~{N}-(1~{H}-indazol-5-yl)butane-1-sulfonamide | C11 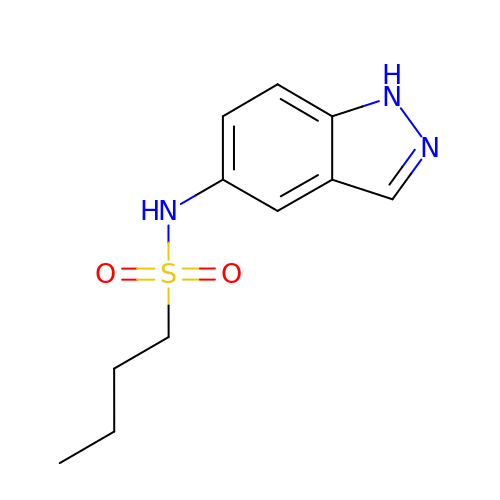H15 N3 O2 S | OPXDHLZGQKADDC-UHFFFAOYSA-N> GRDLRDNETWWYNPSIIVHPHWREFDQVPDAVYYSLGIFIGICGIIGCGGNGIVIYLFTKTKSLQTPANMFIINLAFSDFTFSLVNGFPLMTISCFLKKWIFGFAACKVYGFIGGIFGFMSIMTMAMISIDRYNVIGRPMAASKKMSHRRAFIMIIFVWLWSVLWAIGPIFGWGAYTLEGVLCNCSFDYISRDSTTRSNILCMFILGFFGPILIIFFCYFNIVMSVSNHEKEMAAMAKRLNAKE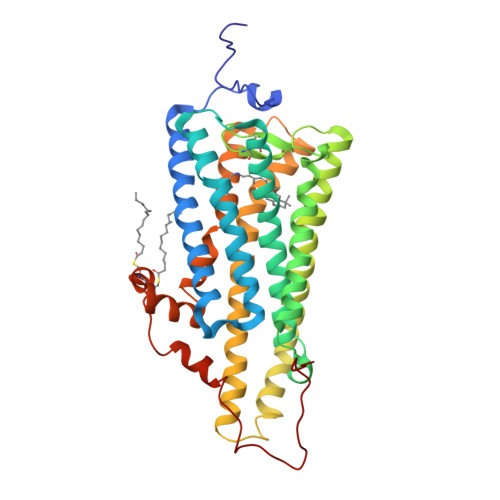LRKAQAGANAEMRLAKISIVIVSQFLLSWSPYAVVALLAQFGPLEWVTPYAAQLPVMFAKASAIHNPMIYSVSHPKFREAISQTFPWVLTCCQFDDKETEDDKDAETEIPAGESSDAAPSADAAQMKE>[2x]GSHPFDQAVVKDPTASYVDVKARRTFLQSGQLDDRLKAALPKEYDCTTEATPNPQQGEMVIPRRYLSGNHGPVNPDYEPVVTLYRDFEKISATLGNLYVAT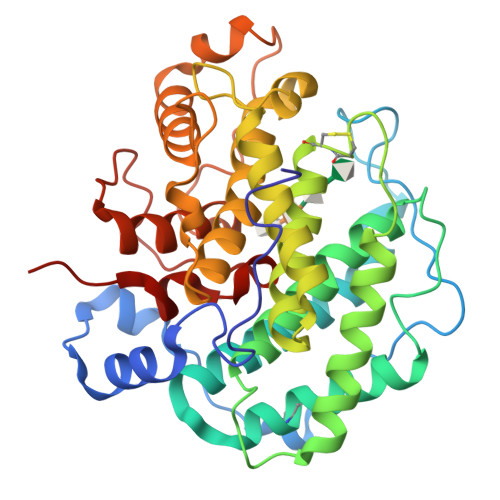GKPVYATCLLNMLDKWAKADALLNYDPKSQSWYQVEWSAATAAFALSTMMAEPNVDTAQRERVVKWLNRVARHQTSFPGGDTSCCNNASYWRGQEATIIGVISKDDELFRWGLGRYVQAMGLINEDGSFVHEMTRHEQSLHYQNYAMLPLTMIAETASRQGIDLYAYKENGRDIHSARKFVFAAVKNPDLIKKYASEPQDTRAFKPGRGDLNWIEYQRARFGFADELGFMTVPIFDPRTGGSATLLAYKPQG>GPLGSQSAKIKLDAPTTRTTCTNNSFKQFDASFSFNEVELTKVETKGGTFASVSIPGAFPTGEVGSPEVPAVRKLIAVPVGATPVVRVKSFTEQVYSLNQYGSEKLMPHQPSMSKSDDPEKVPFVYNAAAYARKGFVGQELTQVEMLGTMRGVRIAALTINPVQYDVVANQLKVRNNIEIE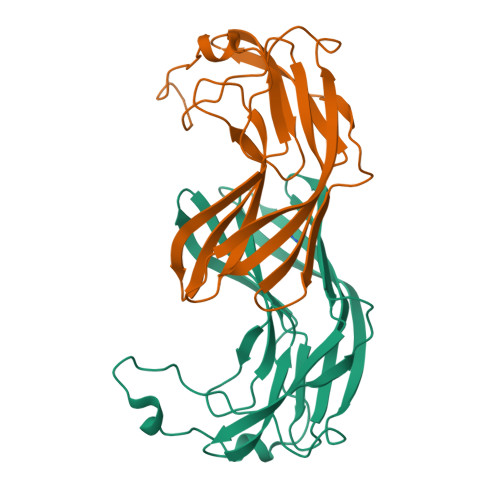VSFQGADEVATQRLYDASFSPYFETAYKQLFNR[2x]>MARAYTDPILFGAAYYDEYIPRDLDRIDTDMEMMTRAGINVIRIGESTWSTCEPQPGHFDWTHIDRALDAATNAGINVIVGTPTYAVPTWLVAMYPDVLATTPAGEPHYGARQIMNIVNPAYRLYGERVIRSLISHVAQQPCVIGYQVDNETKYYDSVSHDMQVMFIKQLRHEFKNDLEALNEAYGLDYWSNRINAWEDFPDLTGSINESLRARFDRFRRDQVAEYLAWQASIIREYMRDDQFITHNFDYEWRGHSYGLQPAVDHFRAARALDICGVDIYHPSEDALTGKEIAFGGDMARSAGGGNYLVLETQAQGQHGWLPYPGQLRLQAYSHLASGADGIMYWHWHSIHNSFETYWRGLLSHDFESNPTYEEAGRFGREIGDPRIGDTLSHLSKRNAVAILASNESLTALSWFHIETGFPMGGTLTYNDVLRSIYDALFELNVEVDFLPADASADQLAGYSLVIAPALYTTDQQTIDRLARYVKNGGHLLATMRSFVADENVKVWHDKAPHHLVDIFGMTYNQFTRPMGVSLKCPDTLADLAG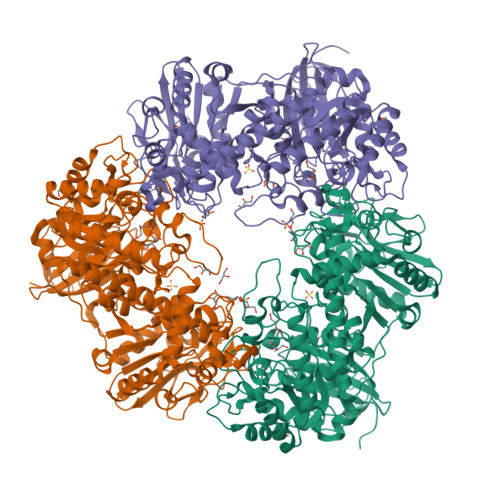ASANDFIEMLSPAPETHVLAWYDHYAWDSYAAITRHAFGSGDAQWVGTQLQADAWRTVLAEALSNAGVHTPGMELAGTVCVRSGTNTAGDTVTYLLNYSGSPITFRAPASGTFLLGHPTDDGEQAVTAETPVTVGDAVTLPRWGVDIIVGRQPTMNAAALEHHHHHH[6x]> DAASDLKSRLDKVS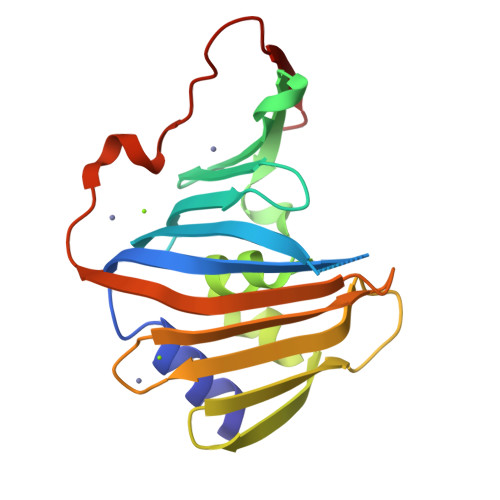SFHASFTQKVTDGSGAAVQEGQGDLWVKRPNLFNWHMTQPDESILVSDGKTLWFYNPFVEQATATWLKDATGNTPFMLIARNQSSDWQQYNIKQNGDDFVLTPKASNGNLKQFTINVGRDGTIHQFSAVEQDDQRSSYQLKSQQNGAVDAAKFTFTPPQGVTVDDQRK> GEIQWMRPSKEVGYPIINAPSKTKLEPSAFHYVFEGVKEPAVLTKNDPRLKTDFEEAIFSKYVGNKITEVDEYMKEAVDHYAGQLMSLDINTEQMCLEDAMYGTDGLEALDLSTSAGYP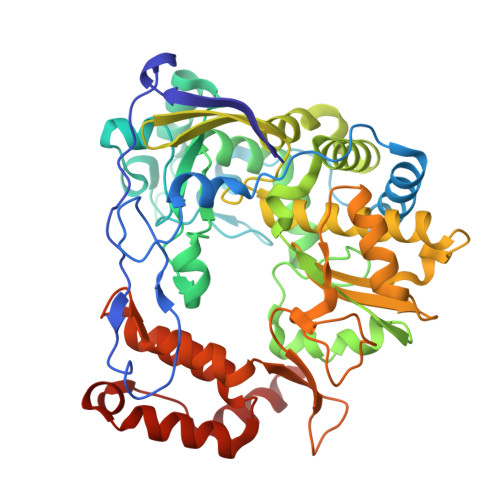YVAMGKKKRDILNKQTRDTKEMQKLLDTYGINLPLVTYVKDELRSKTKVEQGKSRLIEASSLNDSVAMRMAFGNLYAAFHKNPGVITGSAVGCDPDLFWSKIPVLMEEKLFAFDYTGYDASLSPAWFEALKMVLEKIGFGDRVDYIDYLNHSHRLYKNKTYCVKGGMPSGCSGTSIFNSMINNLIIRTLLLKTYKGIDLDHLKMIAYGDDVIASYPHEVDASLLAQSGKDYGLTMTPADKSATFETVTWENVTFLKRFFRADEKYPFLIHPVMPMKEIHESIRWTKDPRNTQDHVRSLCLLAWHNGEEEYNKFLAKIRSVPIGRALDLPEYSTLYDRWLDSF> MAMKNKVQLITYADRLGDGTIKSMTDILRTRFDGVYDGVHILPFFTPFDGADAGFDPIDHTKVDERLGSWDDVAELSKTHNIMVDAIVNHMSWESKQFQDVLAKGEESEYYPMFLTMSSVFPNGATEEDLAGIYRPRPGLPFTHYKFAGKTRLVWVSFTPQQVDIDTDSDKGWEYLMSIFDQMAASHVSYIRLDAVG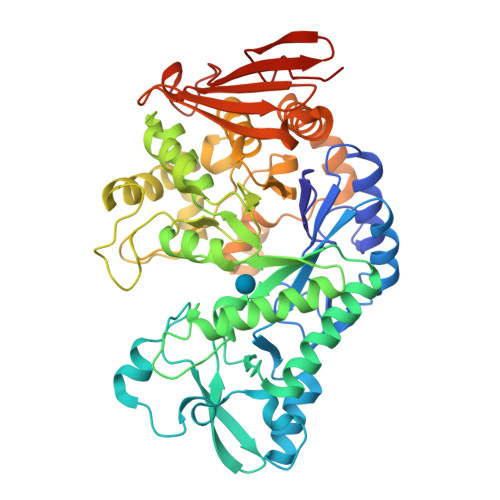YGAKEAGTSCFMTPKTFKLISRLREEGVKRGLEILIEVHSYYKKQVEIASKVDRVYDFALPPLLLHALSTGHVEPVAHWTDIRPNNAVTVLDTHDGIGVIDIGSDQLDRSLKGLVPDEDVDNLVNTIHANTHGESQAATGAAASNLDLYFVNSTYYSALGCNDQHYIAARAVQFFLPGVPQVYYVGALAGKNDMELLRKTNNGRDINRHYYSTAEIDENLKRPVVKALNALAKFRNELDAFDGTFSYTTDDDTSISFTWRGETSQATLTFEPKRGLGVDNTTPVAMLEWEDSAGDHRSDDLIANPPVVALEHHHHHH METHYL N-[(2S,3R)-3-AMINO-2-HYDROXY-3-(4-ISOPROPYLPHENYL)PROPANOYL]-D-ALANYL-D-LEUCINATE | C22 H35 N3 O5 | 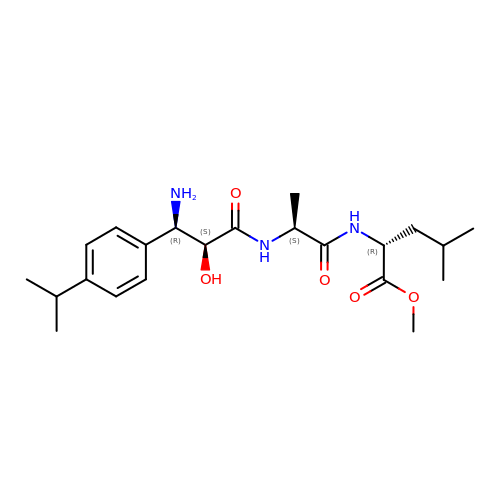WIWZNHHLFMPGGO-PIKADFDJSA-N>MQVKPCTPEFYQTHFQLAYRLQSRPRGLALVLSNVHFTGEKELEFRSGGDVDHSTLVTLFKLLGYDVHVLCDQTAQEMQEKLQNFAQLPAHRVTDSCIVALLSHGVEGAIYGVDGKLLQLQEVFQLFDNANCPSLQNKPKMFFIQACRGDETDRGVDQQD[2x];>[2x]GKEKLPKMRLPTRSDMICGYACLKGTAAMRNTKRGSWYIEALAQVFSERACDMHVADMLVKVNALIKDREGYAPGTEFHRCKEMSEYCSTLCRH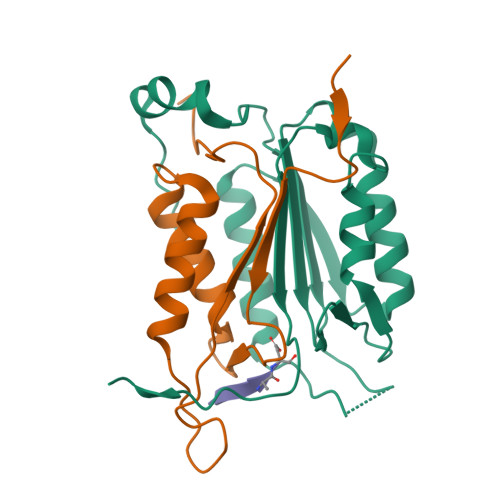LYLFPGHPPTLEHHHHHH;>[2x]XVDVAD>[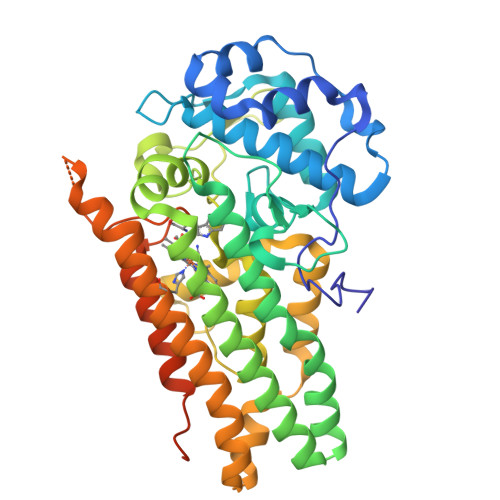2x]MSKEYHIDEEVGFALPNPQENLPDFYNDWMFIAKHLPDLIESGQLRERVEKLNMLSIDHLTDHKSQRLARLVLGCITMAYVWGKGHGDVRKVLPRNIAVPYCQLSKKLELPPILVYADCVLANWKKKDPNKPLTYENMDVLFSFRDGDCSKGFFLVSLLVEIAAASAIKVIPTVFKAMQMQERDTLLKALLEIASCLEKALQVFHQIHDHVNPKAFFSVLRIYLSGWKGNPQLSDGLVYEGFWEDPKEFAGGSAGQSSVFQCFDVLLGIQQTAGGGHAAQFLQDMRRYMPPAHRNFLCSLESNPSVREFVLSKGDAGLREAYDACVKALVSLRSYHLQIVTKYILIPASQQPKENKTSEDPSKLEAKGTGGTDLMNFLKTVRSTTEKSLLKEGKGELNSKLEGKPIPNPLLGLDSTRTGHHHHHH> MQEIALTPQPAHLTVKDGRFEFGNQLKAKVTPYQGDS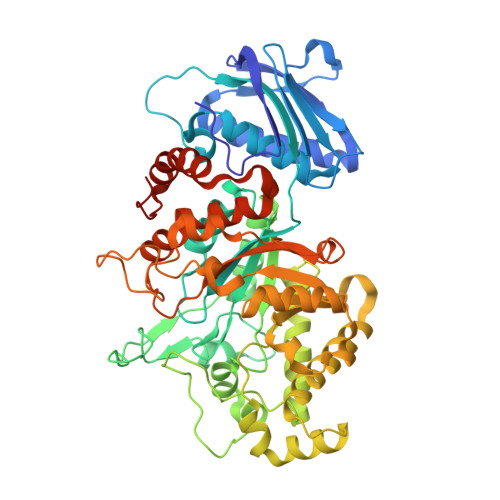IRMVFESFKKELQEATGIKVSSTQKEAKARIILDLNPQLPAEAYKLNVSKKQVRIEASRPAGFYYALQTLKQLMPRNVMAGVATSDHSQWSLPSVEIEDAPRFEWRGFMLDEGRHFFGKDEIKRVIDMMAIYKMNRFHWHLTEDQGWRIEIKKYPKLTETGAWRNSKVLAYGDVKPDGERYGGFYTQKDIKEIVAYAKKKFIEIIPEIDIPGHSQAAVAAYPEFLACDPRDKHEVWLQQGISTDVINVANPKAMQFAKEVIDELTELFPFNYIHLGGDECPTRKWQKNDECKKLLSEIGSSNFRDLQIYFYKQLKDYIATKPADQQRQLIFWNEVLHGNTSILGNDITIMAWIGANAAAKQAAKQGMNTILSPQIPYYINRKQSKLPTEPMSQGHGTETVEAVYNYQPLKDVDAALQPYYKGVQANFWTEWVTEPSVLEYLMLPRLAAVAEAGWTPQEKRNYEDFKERIRKDAELYDLKGWNYGKHIMKLEHHHHHH Bacteriophage exclusion (‘BREX’) systems are multi-protein complexes encoded by a variety of bacteria and archaea that restrict phage by an unknown mechanism. The final gene in most type 1 BREX systems, termed ‘BrxL’, encodes a large protein (670–700 residues in various species), with much of its sequence predicted to adopt a fold corresponding to the chambered ATP-dependent AAA+ protein family, which are involved in a wide variety of cellular functions throughout all biological kingdoms. In this study we have demonstrated that the BrxL phage restriction factor is a multimeric DNA binding protein that displays ATP-dependent assembly on double stranded DNA.

To study the structure of full-length BrxL we next purified two constructs, wild-type BrxL (BrxLWT) and a variant containing a catalytic point mutation in the ATPase ‘Walker B’ catalytic motif (BrxLE280Q). Grids generated using BrxLE280Q also displayed a mixture of partially and fully assembled protein complexes, with the latter displaying protrusions from each end of the long axis of the complex. A subsequent CryoEM structure determination of full-sized particles produced electron density maps extending to ∼3 Å resolution that correspond to dodecameric particles comprising two six-fold symmetric (hexameric) protein rings, again associated with one another in an antiparallel tail-to-tail arrangement. In addition to the difference in protein copy number and symmetry between the unbound versus DNA-bound BrxL protein assemblages (corresponding to two heptamers versus two hexamers), the BrxLE280Q density maps also demonstrated the unambiguous presence of double stranded DNA spanning the length of the BrxL chamber, which would seem likely to represent DNA from the bacterial expression host that was bound by BrxL during expression and/or cell lysis and then carried through the purification process. The density of the DNA was not of sufficient resolution to directly determine a specific sequence of the bound DNA moiety, and so the modeled identity of bases in the refined model represents an arbitrary sequence based on the best fit to density at each position. Approximately 6 full turns of DNA (62 basepairs) were visible and modeled into the density. The dimensions of the BrxL (E280Q) dodecamer are ∼195 Å in the longest dimension and 140 Å across the exterior diameter of the cylinder. The diameter of the interior chamber is narrowest (∼30 Å) at each end of the protein assemblage, where positively charged loop regions from the NTD and AAA+ ATPase domains of each subunit are in closest contact with the DNA, and considerably wider (∼80 Å) near the chamber's equator, where the C-terminal domain of each subunit makes contacts with the same domain in the opposing protein hexameric ring. Multiple contacts to the DNA backbone, at each end of the bound duplex, are contributed by basic residues extending from loops contributed by the NTD and the AAA+ domains.

>MESANDKELDQLLNEHFAGRVVRKDLTKLIKEGANVPVYVLEYLLGMYCASDDPEIIEQGLRNVKTVLAENYVRPDEAEKVKSLVRERGSYKVIDRVTVKLNERKDKYEASFSNLGIKDAEISAGIVKEYEKLLVGGIWVIATLSYYFEEGQTSSPFGVSLLKPIQMPNMNMDELFSGRAALSTDQWRESLIRSIGMEPASLKEDVQWHLLARMVPFVENNYNVCELGPRGTGKSHIYKECSPNSILVSGGQTTVANLFYNMSSRRIGLVGLWDVVAFDQVAGISFKDKDGVQIMKDYMASGSFARGREQMEASASMVFVGNINQSVESLVKTSHLLAPFPEAMIDSAFFDRFHAYIPGWEIPKMRPEFFTNRYGLIVDYLAEFFREMRKRSFADSIEKYFKLGNNLNQRDVIAVRKTVSGLMKLLYPHGQFNKEDVRQCLEYALQVRRRVKEQLKKIGGMEFYDVHFSYIDNDTLEEHFVSVKEQGGGGLIPEGPAKPGFLYTIGLSNKGMPGLYRLELQVTKGSGKLATSGLWNSSSAKEQVKIAFDYFKANASRISGGSKVMEHDFHLHVVELQNTGPLSHLALPSLVAFASGLLGRSVQSQMVVLGDMSLGGSVTPVESIAECLQVAFDAGAKKVALPMSSAADIPTIPVELFTKFQTSFYADPVDAVFKGLGVD[12x]> MNFNVSLMEKLKWKIKCIENKFLNYRLTTNETVVAETEYGKVKGVKRLTVYDDSYYSFEGIPYAQPPVGELRFKAPQRPTPWDGVRDCCNHKDKSVQVDFIAGKVCGSEDCLYLSVYTNNLNPETKRPVLVYIHGGDFIIGENHRDMYGPDYFIKKDVVLINIQYRLGA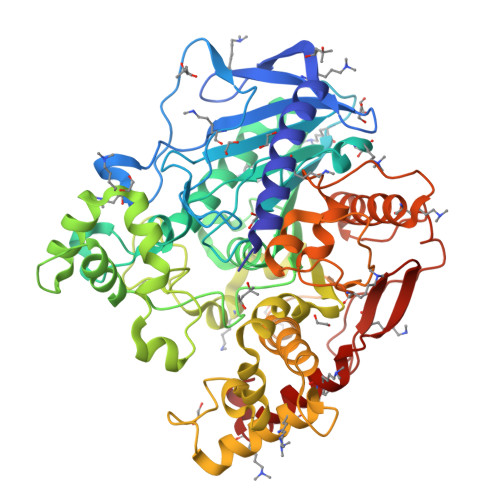LGFLSLNSEDLNVPGNAGLKDQVMALRWIKNNCANFGGNPDNITVFGESAGAASTHYMMLTEQTRGLFHRGILMSGNAICPWANTQCQHRAFTLAKLAGYKGEDNDKDVLEFLMKAKPQDLIKLEEKVLTLEERTNMVVFPFGPTVEPYQTADCVLPKHPREMVKTAWGNSIPTMMGNTSYEGLFFTSILKQTPMLVKELETCVNFVPSELADAERTAPETLEMGAKIKKAHVTGETPTADNFMDLCSHIYFWFPMHRLLQLRFNHTSGTPVYLYRFDFDSEDLINPYRIMRSGRGVKGVSHADELSYFFWNQLAKRMPKESREYKTIERMTGIWIQFATTGNPYSNEIEGMENVSWDPIKKSDEVYKCLNISDELKMIDVPEMDKIKQWESMFEKHRDLF> FDNSTLGTPTTHVSMKKKESENDSEQQLNFPPDRTDEIRKTIQHDVETNAAFQNPLFNDELKYWLDSKRYLMQPLQEMSPKMVSQLESSLLNCPDSLDADSPCLYTKPLSLPHPTSIFFPNEPIRF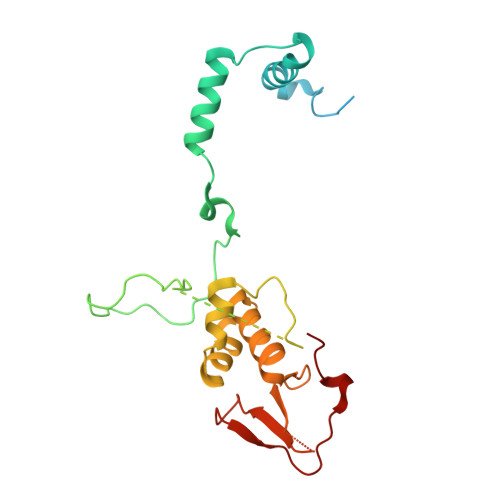VYPYDVPLNLTNNENDTDNKFGKDSKAKSKKDDDIYSRTSLARIFMKFDLDTLFFIFYHYQGSYEQFLAARELFKNRNWLFNKVDRCWYYKEIEKLPPGMGKSEEESWRYFDYKKSWLARRCGNDFVYNEEDFEKL>MNSSKETKSEPSDSKKLMDQPYSKTDFLMGTVVTLKIYDKGKEDVLDKGFDRIKDLAAKITTSDSEKTSEVDKINEQA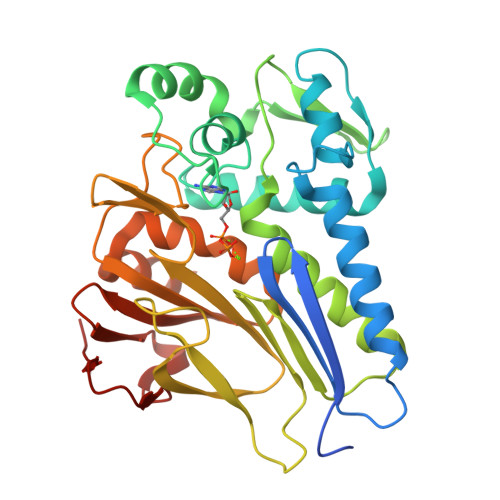GKKPVKVSEDVYYLIQEGLKYSENSGGSFDITIGPLTSLWHIGFSDARKPSQAEIDAVLPLINYKDVKMNDKDQTVYLEKEGMELDLGAIAKGFITDETLKVFKENKVTTSIIDLGGNIYVQGNNPNGNKWNVGIQDPFSPRGSVIGKLPESNMSIVTSGIYERYLEVDGKTYHHILDPKTGYPFDNDIAGVSIVSKKSIDGDGLSTATFSKGIKGGMDYIEQFEGVDAIFISKEKKVYETSGLKGQFELTDKDFQMDTLKK[2x]> HMKNYLRVVGNMEARFAVATPEELAVNNDDCAICWDSMQAARKLPCGHLFHNSCLRSWLEQDTSCPTCRMSLNIADNNRVREEGGGGGGGSSGS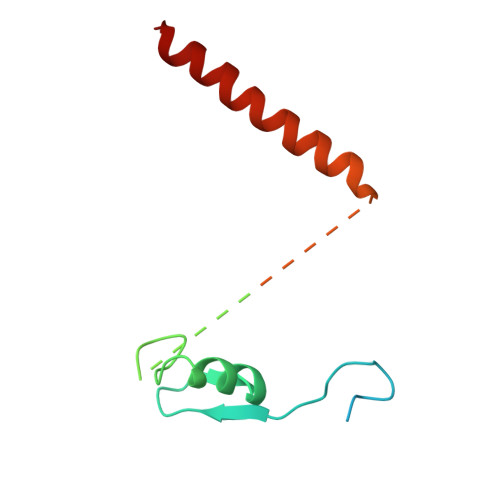SGGSGGGSGSSSGGGGGSGGGSGGGGGGGSADERQRMLVQRKDELLQQARKRFLNK>HGYIDSPGSRAFLCSAQGNEQNMDCGLVKYEPQSLEAKKGFPQAGPEDGHIASAGIGHFGALDAQTEDRWKKIPITAGE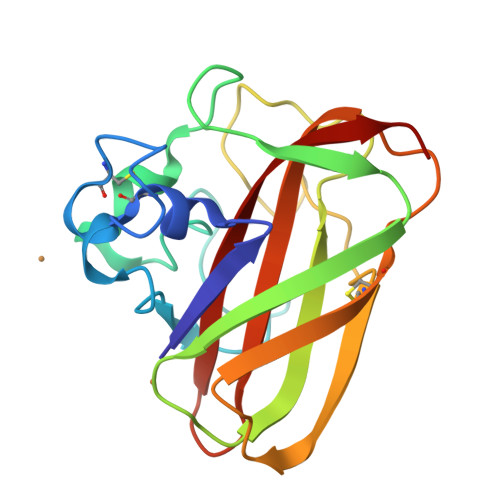IEFQWEIMIQHKTSSWEYFITKLGWDPNKPLTREQFNSTPFCFEDYQEKMPSSRVINKCTLPEGYQGYHVILGVWTISDTLNAFYQVIDTTISPA[3x]(2~{S},3~{S})-~{N}-[(2-methoxyphenyl)methyl]-2-phenyl-piperidin-3-amine | C19 H24 N2 O | 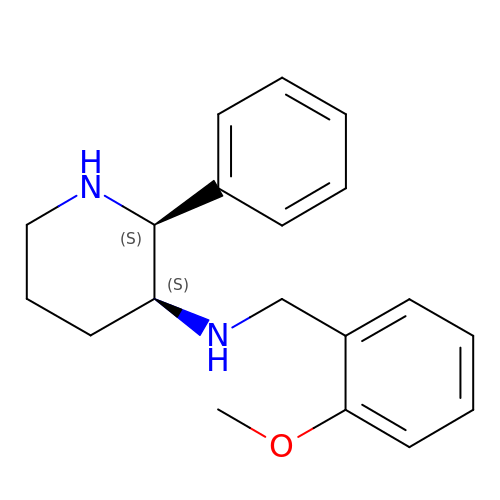DTQNEFOKTXXQKV-HKUYNNGSSA-N>MNVIAILNHMGVYFKEEPIRELHRALERLNFQIVYPNDRDDLLKLIENNARLCGVIFDWDKYNLELCEEISKMNENLPLYAFANTYSTLDVSLNDLRLQISFFEYALGAAEDIANKIKQTTDEYINTILPPLTKALFKYVREGKYTFCTPGHMGGTAFQKSPVGSLFYDFFGPNTMKSDISISVSELGSLLDHSGPHKEAEQYIARVFNADRSYMVTNGTSTANKIVGMYSAPAGSTILIDRNCHKSLTHLMMMSDVTPIYFRPTRNAYGILGGIPQSEFQHATIAKRVKETPNATWPVHAVITNSTYDGLLYNTDFIKKTLDVKSIHFDSAWVPYTNFSPIYEGKCGMSGGRVEGKVIYETQSTHKLLAAFSQASMIHVKGDVNEETFNEAYMMHTTTSPHYGIVASTETAAAMMKGNAGKRLINGSIERAIKFRKEIKRLRTESDGWFFDVWQPDHIDTTECWPLRSDSTWHGFKNIDNEHMYLDPIKVTLLTPGMEKDGTMSDFGIPASIVAKYLDEHGIVVEKTGPYNLLFLFSIGIDKTKALSLLRALTDFKRAFDLNLRVKNMLPSLYREDPEFYENMRIQELAQNIHKLIVH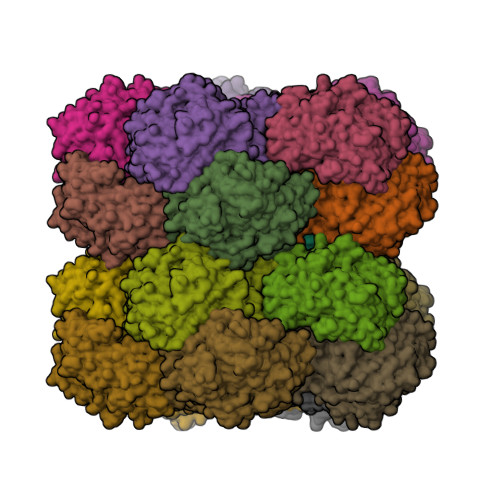HNLPDLMYRAFEVLPTMVMTPYAAFQKELHGMTEEVYLDEMVGRINANMILPYPPGVPLVMPGEMITEESRPVLEFLQMLCEIGAHYPGFETDIHGAYRQADGRYTVKVLKE[20x]Human endonuclease VIII-like 1 (hNEIL1) is a bifunctional DNA glycosylase of the Fpg/Nei family, which catalyzes the removal of damaged bases and subsequent incision of the newly generated abasic sites. Unlike traditional enzymes which are commonly referred to as highly specific biocatalysts, one special feature for hNEIL1 is its unique capability to recognize a wide range of substrates, including formamidopyrimidines, hydantoin lesions, oxidized, and dihydro-modified pyrimidine bases, derived from all four canonical bases. Here, by integrating structural, computational, and biochemical investigations, we show that hNEIL1 uses a triage mechanism to achieve broad specificity and reduce futile repair of normal bases. This mechanism involves two mutually competing interaction states: an activated state that commits catalysis and BER, and a quarantine state that temporarily separates and prevents the flipped base from catalysis via auto-inhibition.

We synthesized a 2′-fluoro-substituted stable mimic of DHU (FDHU), which allows binding but not catalysis by hNEIL1. By undergoing a base–acid equilibrium with the adjacent Glu6, K242 can interact with the flipped base as a hydrogen bond acceptor (denoted as “Tau-K2”), forgoing the pre-requisite of the base-tautomerization (“Tau-K1”). Through QM/MM calculations we found that, due to the moderate basicity of K242 (pKa~10), “Tau-K2” is indeed a stable configuration of the activated state in addition to the base-tautomerized “Tau-K1”. Accordingly, K242 is more likely to retain the base in the activated state compared to R242, or in other words, the activated state is more favored by the genomically encoded hNEIL1(K242) compared to its RNA-edited counterpart, which is supported by our QM/MM calculations. Indeed, these two forms of hNEIL1 have been shown to have different glycosylase activities where the unedited hNEIL1(K242) is faster than edited hNEIL1(R242) on several substrates.

>[3x]MPEGPELHLASQFVNEACRALVFGGCVEKSSVSRNPEVPFESSAYRISASARGKELRLILSPLPGAQPQQEPLALVFRFGMSGSFQLVPREELPRHAHLRFYTAPPGPRLALCFVDIRRFGRWDLGGKWQPGRGPCVLQEYQQFRENVLRNLADKAFDRPICEALLDQRFFNGIGNYLRAEILYRLKIPPFEKARSVLEALQQHRPSPELTLSQKIRTKLQNPDLLELCHSVPKEVVQLGGKGYGSESGEEDFAAFRAWLRCYGMPGMSSLQDRHGRTIWFQGDPGPLAPKGRKS>[3x]MHPKIFALLAKFPRVELIPWETPIQYLPNISREIGADVYIKRDDLTGLGIGGNKIRKLEYLLGDALSKGADVVITVGAVHSNHAFVTGLAAKKLGLDAILVLRGKEELKGNYLLDKIMGIETRVYDAKDSFELMKYAEEIAEELKREGRKPYVIPPGGASPIGTLGYVRAVGEIATQSEVKFDSIVVAAGSGGTLAGLSLGLSILNEDIRPVGIAVGRFGEVMTSKLDNLIKEAAELL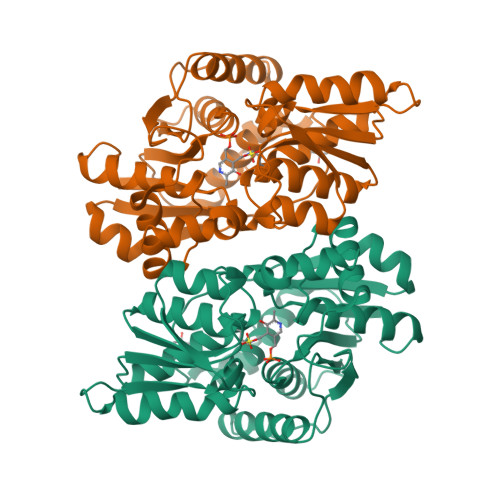GVKVEVRPELYDYSFGEYGKITGEVAQIIRKVGTREGIILDPVYTGKAFYGLVDLARKGELGEKILFIHTGGISGTFHYGDKLLSLL>[4x]HHHHAYYSMYLKEIFVDNFRNLKKQKLEFCEGVNLIYGLNAQGKSNLLEAIRLLSMGRSFRGSKMSELVKFDEEYFYVRGLVRSADFYEKKIEFGYKVNGNKVIKVNGNKLKSTGEILGHFLTVIFSPEDIEIIKEGPSRRRKYLDACISVIDKNYFFDLLQYNKTLSNRNSLLKKIKEEGKGEDLLEIFDEKLAEYGARIIKVRNNYLEKLKNSMSKFLMEISNEKLEIIYLNSAGVKEVHEENLIREKLKNRLTKSLTLDLKYLSTQVGPHREDFKILINGYDSRVYSSQGQKRTAALCLKLSELEILEEETGEKPVLLLDDVMSELDDNRKKYILKKLEGFQSFITHTSKSDVEGDCCFKIYDGIVDKLA

RecF is a multifunctional protein involved in recombinant DNA repair, homologous genetic recombination, and DNA replication. Similar to RecR and RecO, RecF is a recombination mediator protein (RMP) in the RecFOR pathway for ssDNA gap repair. RecF contains the conserved Walker A motif, Walker B motif and signature motif of ABC-ATPase that exhibits ATP-dependent dimerization; additionally, the signature motif residues interact with the ATP bound to the opposite molecule. To gain insight into the mechanism of ABC-ATPase RecF, we solved the crystal structures of TTERecF, TTERecF-ATP, and TTERecF-ATPɤS.

We determined the crystal structure of the TTERecF-ATP complex at 3.0 Å through molecular replacement by using TTERecF monomer as a model. In the TTERecF-ATP structure, four RecF monomers formed two dimers in the asymmetric unit. For each stabilized dimer, ATP acted as a fastener that linked domain I of one monomer and domain II of the other monomer and was located between RecF molecules directly opposite to each other. The contact surface area between the two molecules of the dimer was 5863 Å2, which was 17.8% of the total dimer surface area (32919 Å2). In addition, the two long α-helices (αD and αE) of the domain II of two TTERecF formed a channel, within which numerous positive charges and hydrophobic residues were distributed. The diameter of this channel was approximately 20 Å, nearly similar to the dsDNA diameter. Two ATP molecules were buried in the positively charged tunnel of the RecF dimer interface. ATP interacted with the Walker A motif of one TTERecF and with the conserved signature motif of the other TTERecF. Mg2+ in the active site binded to ATP β- and ɤ-phosphate O’s and two H2O molecules. The TTERecF-ATP dimer structure displayed the closed reaction state of TTERecF for interacting with ATP and even for the complex interaction with DNA.>[2x]GSMANKPMQPITSTANKIVWSDPTRLSTTFSAS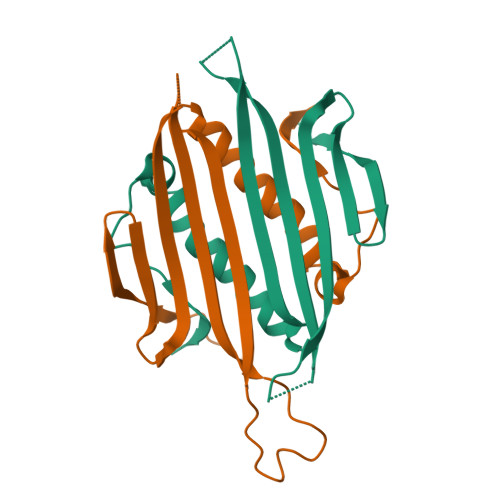LLRQRVKVGIAELNNVSGQYVSVYKRPAPKPEGGADAGVIMPNENQSIRTVISGSAENLATLKAEWETHKRNVDTLFASGNAGLGFLDPTAAIVSSDTTA> MADHNPDSDSTPRTLLRRVLDTADPRTPRRPRSARAGARRALLETASPRKLSGQTRTIARGRSHGARSVGRSAHIQASGHLEEQTPRTLLKNILLTAPESSILMPESVVKPVPAPQAVQPSRQESSCGSLELQLPELEPPTTLAPGLLAPGRRKQRLRLSVFQQGVDQGLSLSQEPQGNADASSLTRSLNLTFATPLQPQSVQRPGLARRPPARRAVDVGAFLRDLRDTSLAPPNIVLEDTQPFSQPMVGSPNVYHSLPCTPHTGAEDAEQAAGRKTQSSGPGLQKNSPGKPAQFLAGEAEEVNAFALGFLSTSSGVSGEDEVEPLHDGVEEAEKKMEEEGVSVSEMEATGAQGPSRVEEAEGHTEVTEAEGSQGTAEADGPGASSGDEDASGRAASPESASSTPESLQARRHHQFLEPAPAPGAAVLSSEPAEPLLVRHPPRPRTTGPRPRQDPHKAGLSHYVKLFSFYAKMPMERKALEMVEKCLDKYFQHLCDDLEVFAAHAGRKTVKPEDLELLMRRQGLVTDQVSLHVLVERHLPLEYRQLLIPCAYSG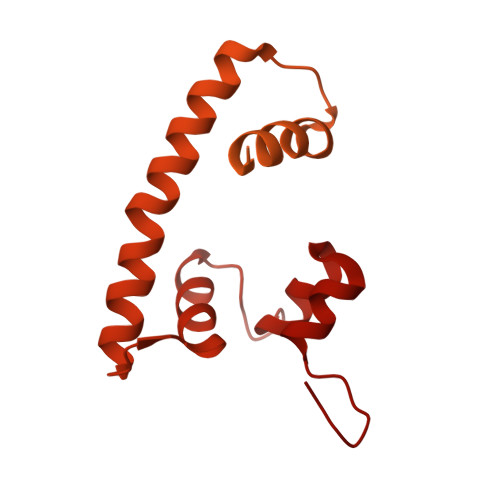NSVFPAQ>[4x]MAESQDKYTRRTGRTWAD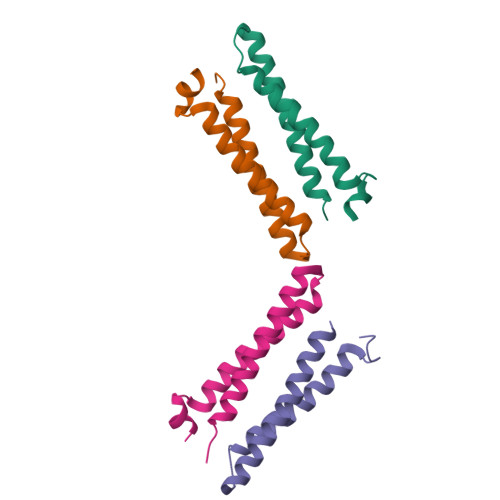DQATYNRLREEADAARQKLRESGYSGAEYDQLRQAAFDLNRKANQYWEQMLSDLRQED> G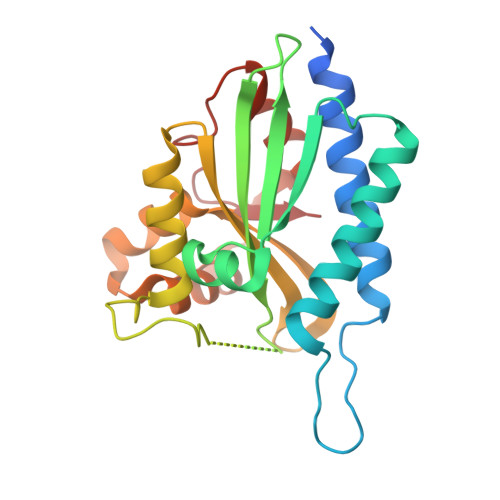HMGQKASQQLALKDSKEVPVVCEVVSEAIVHAAQKLKEYLGFEYPPSKLCPAANTLNEIFLIHFITFCQEKGVDEWLTTTKMTKHQAFLFGADWIWTFWGSDKQIKLQLAVQTLQMSSPPPVESKPCDLSNPESRVEESSWKKSRFDKLEEFCNLIGEDCLGLFIIFGMPGKPKDIRGVVLDSVKSQMVRSHLPGGKAVAQFVLETEDCVFIKELLRNCLSKKDGLREVGKVYISIL>GPGSMNERLEDIALTLVGAGKGILAADESTATIGKRFESIGVECTEDNRRAYREMLFTAKEAMESAISGVILFDETLRQKASTGQMLTDLIRDAGAVPGIKVDTGAKPLAAFPQETITEGLDGLRERLKDYYTLGARFAKWRAVIAIDAQTLPTRGAISQNAQALARYAALCQEAGLVPIVEPEVLMDGPSRQHSITRCFEVTKVVLHTVFKELFEARVLFEGMILKPNMVIDGKDARIASVEEVAEKTVHVLKQTVPAAVPGIAFLSGGQTDEEATAHLSAMNALGALPWKLTFSYGRALQAAALKAWAGKNENIVVAQKAFCHRARMNHLAALGQWTKDQEKSCA[4x]

The glycolytic enzyme fructose bisphosphate aldolase (EC 4.1.2.13) catalyzes the aldol cleavage of fructose 1,6-bisphos­phate into dihydroxyacetone phosphate and glyceraldehyde 3-phosphate. It also catalyzes the reverse reaction. The hallmark of a class I aldolase is the presence of an active-site lysine residue which forms a Schiff base with the substrate. The structure shares the typical barrel tertiary structure and tetrameric quaternary structure reported for previous FBPA structures and exhibits the same Schiff base in the active site.

Here, we present the crystal structure of the class I fructose bisphosphate aldolase from B. henselae with the reactant bound at the active site. The purified enzyme crystallized in the apo form but failed to diffract; however, well diffracting crystals could be obtained by cocrystallization in the presence of the native substrate fructose 1,6-bisphosphate. The final FBP-bound model contains four copies of FBPA including three residues of the four-residue N-terminal purification tag and residues 1–340 (of 343) of the protein; the FBP ligand was modelled in each monomer. Here, we determined the 2.35 Å resolution crystal structure of BhFBPA. This structure has clear electron density for FBP bound at the active site. There is a covalent bond between C atom C2 of the linear FBP molecule and the Nζ atom of Lys223 of the protein. Furthermore, phosphate group 1 of FBP makes hydrogen bonds to three amide N atoms as well as the side chains of Arg295 and Ser264. The alcohol groups along the linear carbon backbone of FBP also make hydrogen bonds to the side chains of the protein, as well as to nearby water molecules. Finally, the O atoms of phosphate group 2 are hydrogen bonded to side chains and to nearby water molecules. We compared the active site of BhFBPA with those of homologous mammalian enzymes. The similarity to the active site of mammalian FBPA A suggests that the design of a specific inhibitor for BhFBPA (that does not inhibit the human enzyme) would be exceptionally challenging and would have to rely on exploiting very minor differences in the chemical environment in and near the active site.>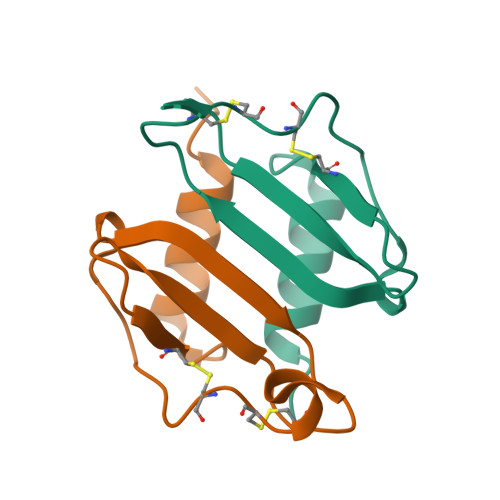[4x]AVVASELRCQCLKTLPRVDFKNIQSLSVTPPGPHCAQTEVIATLKGGQKVCLDPEAPLVQKIIQKILNKGKAN3-(2-hydroxyphenyl)-9H-pyrrolo[2,3-b:5,4-c']dipyridine-6-carbonitrile 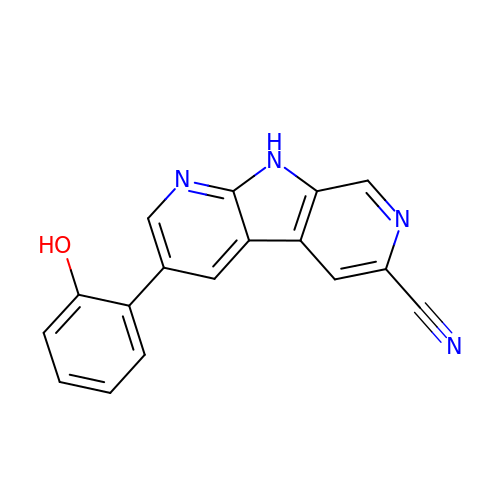| C17 H10 N4 O | NMTUQTHXOJLRMZ-UHFFFAOYSA-N In this work, we exhaustively probe the ability of all 36 immobile HJ sequences to form DNA crystals in two different designed systems. Three separate self-assembling DNA crystal systems are described in this report: the “4 × 5” and “4 × 6” designs (collectively referred to as the 4 × N systems), and a third construct with a “scrambled” sequence variant of the 4 × 6 lattices. Self-assembly was mediated by three constituent oligonucleotides: (S1) containing four sequence repeats of either 5 or 6 bases; (S2) composed of 21 bases containing complementary regions to both (S1); and (S3) which forms the second junction crossover. The HJ serves as the fundamental component at the core of each unit, and the ultimate assembly of the full lattice is facilitated by the complementary 2-base sticky ends that tail each duplex.

The 4 × 5 system robustly crystallized with 75% of the junctions, and we obtained crystals in all but 9 of 36 sequences. Of the resulting structures, 18 exhibited P32 symmetry with average cell dimensions a = b = 68.85 Å c = 60.09 Å, with only nine retaining the original P3221 symmetry with average cell edges a = b = 68.17 Å c = 60.60 Å. The P32 channels were treated as a hexagonal prism with 6.4 nm along each edge and a height measured from the top to the bottom of each block along with the average c-axis = 6.0 nm, with a resulting volume of ~639 nm3, a nearly 27-fold increase in cavity size relative to the P3221 lattices. We hypothesize that even a small difference in junction angles could have a significant global effect on the assembly of the lattice, thereby eliminating the strain in the P3221 lattices.

> GAGCAGACGTGACTCCACTCA;> AGTCA;> TCTGAGTGG;> CGTCTGC> MERPISEAYFQEAKRHIPGGVSSPVRAFKAVGGTPPFLVRGEGAYVWDADGNRYLDYVMSWGPLILGHAHPKVLARVRETLERGLTFGAPSPLEVALAKKVKRAYPFVDLVRFVNSGTEATMSALRLARGYTGRPYIVKFRGNYHGHADGLLVEAGSGALTLGVPSSAGVPEEYAKLTLVLEYNDPEGLREVLKRRGEEIAAIIFEPVVGNAGVLVPTEDFLKALHEAKAYGVLLIADEVMTGFRLAFGGATELLGLKPDLVTLGKILGGGLPAAAYAGRREIMEK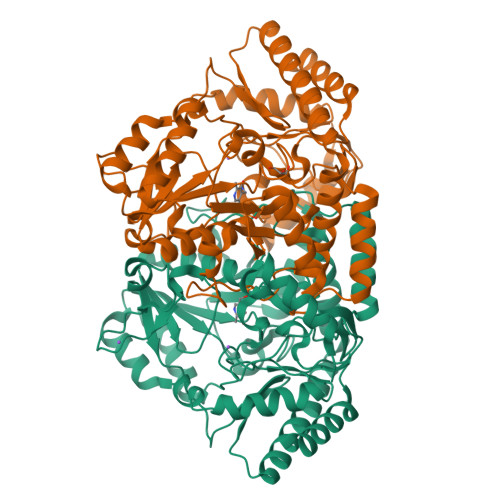VAPLGPVYQAGTLSGNPLAMAAGLATLELLEENPGYYAYLEDLGARLEAGLKEVLKEKGLPHTVNRVGSMITVFFTEGPVVTFQDARRTDTELFKRFFHGLLDRGIYWPPSNFEAAFLSVAHREEDVEKTLEALRKAL>AEFFPEIPKVQFEGKESTNPLAFKFYDPEEIIDGKPLKDHLKFSVAFWHTFVNEGRDPFGDPTADRPWNRYTDPMDKAFARVDALFEFCEKLNIEYFCFHDRDIAPEGKTLRETNKILDKVVERIKERMKDSNVKLLWGT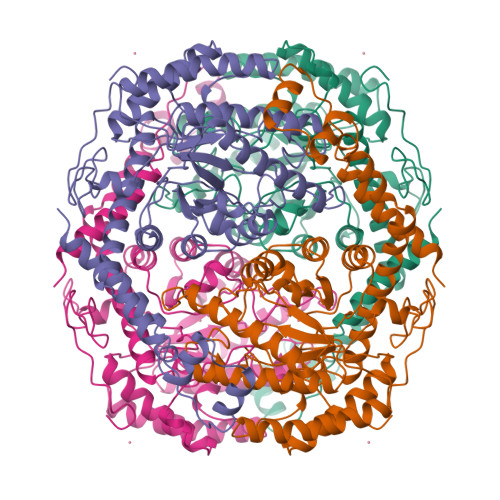ANLFSHPRYMHGAATTCSADVFAYAAAQVKKALEITKELGGEGYVFWGGREGYETLLNTDLGFELENLARFLRMAVDYAKRIGFTGQFLIEPKPKEPTKHQYDFDVATAYAFLKSHGLDEYFKFNIEANHATLAGHTFQHELRMARILGKLGSIDANQGDLLLGWDTDQFPTNVYDTTLAMYEVIKAGGFTKGGLNFDAKVRRASYKVEDLFIGHIAGMDTFALGFKVAYKLVKDGVLDKFIEEKYRSFREGIGRDIVEGKVDFEKLEEYIIDKETIELPSGKQEYLESLINSYIVKTILELR[2x]>MAPKSSSSGSKKKSSASSNSADAKASKFKLPAEFITRPHPSKDHGKETCTAYIHPNVLSSLEINPGSFCTVGKIGENGILVIARAGDEEVHPVNVITLSTTIRSVGNLILGDRLELKKAQVQPPYATKVTVGSLQGYNILECMEEKVIQKLLDDSGVIMPGMIFQNLKTKAGDESIDVVITDASDDSLPDVSQLDLNMDDMYGGLDNLFYLSPPFIFRKGSTHITFSKETQANRKYNLPEPLSYAAVGGLDKEIESLKSAIEIPLHQPTLFSSFGVSPPRGILLHGPPGTGKTMLLRVVANTSNAHVLTINGPSIVSKYLGETEAALRDIFNEARKYQPSIIFIDQIDSIAPNRANDDSGEVESRVVATLLTLMDGMGAAGKVVVIAATNRPNSVDPALRRPGRFDQEVEIGIPDVDARFDILTKQFSRMSSDRHVLDSEAIKYIASKTHGYVGADLTALCRESVMKTIQRGLGTDANIDKFSLKVTLKDVESAMVDIRPSAMREIFLEMPKVYWSDIGGQEELKTKMKEMIQLPLEASETFARLGISAPKGVLLYGPPGCSKTLTAKALATESGINFLAVKGPEIFNKYVGESERAIREIFRKARSAAPSIIFFDQIDALSPDRDGSSTSAANHVLTSLLNEIDGVEELKGVVIVAATNRPDEIDAALLRPGRLDRHIYVGPPDVNARLEILKKCTKKFNTEESGVDLHELADRTEGYSGAEVVLLCQEAGLAAIMEDLDVAKVELRHFEKAFKGIARGITPEMLSYYEEFALRSGSSS[6x]

The type II AAA + ATPase Drg1 is a ribosome assembly factor, functioning to release Rlp24 from the pre-60S particle just exported from nucleus, and its activity in can be inhibited by a drug molecule diazaborine. Here, we report Drg1 structures in different nucleotide-binding and benzo-diazaborine treated states. All structures display a typical three-layered architecture, similar to those of type II AAA + hexamers, such as p97/VCP and Cdc48, and the NTD, D1, and D2 rings show an apparent deviation from a perfect sixfold symmetry. Comparisons of these structures indicate that Drg1 hexamers transit between two extreme conformations, a planar and a helical state.

Next, we prepared a mutant form of Drg1 with two mutations (E346Q and E617Q) located in Walker B motif of the D1 and D2 domains, respectively. Mutant Drg1 hexamers were incubated with excessive ATP for stable hexamer formation before cryo-EM sample preparation. The cryo-EM structure of mutant Drg1 hexamers was determined at a much-improved resolution of 3.5 Å. Similar as in the structural study of Rix722, the introduction of the Walker B double mutation allowed the capture of an endogenous peptide within the central channel of Drg1 hexamer during purification. In the structure of the mutant Drg1 hexamer (Drg1E346Q/E617Q-ATP), a polypeptide was found in the central channel, which passes through the central pores of Drg1 hexamers formed by the PLs of the D1 and D2 rings. The density of the main chain of this peptide was well resolved such that we could build a poly-alanine model (23 residues) for it. The six protomers of Drg1 form a spiral staircase to accommodate the peptide. Thus, P6 of the mutant Drg1 hexamer should be the “seam” subunit reported in the structures of Cdc48/p97 and Rix7 in substrate-engaged states. Specifically, while the polypeptide is held by PL-Is from four protomers (P2–P5) at the D1 layer, it is clamped by PL-Is from five protomers (P1–P5) at the D2 layer. The D1 domains of all six protomers are in the ATP-bound state, which is similar to the substrate engaged structures of Cdc48 and Rix711,12,22.> SIADYKDDDDKMRAEGLGGLERFCSPGKGRGLRALQPFQVGDLLFSCPAYAYVLTVNERGNHCEYCFTRKEGLSKCGRCKQAFYCNVECQKEDWPMHKLECSPM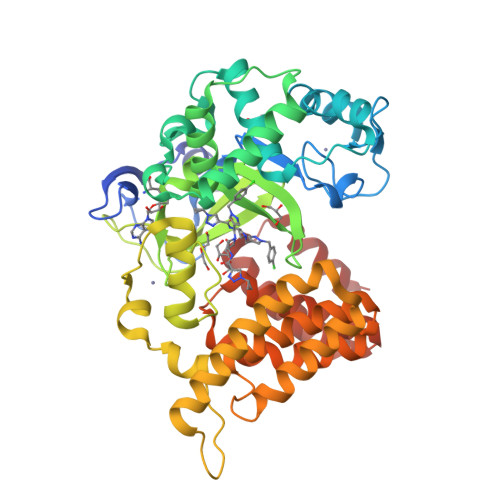VVFGENWNPSETVRLTARILAKQKIHPERTPSEKLLAVKEFESHLDKLDNEKKDLIQSDIAALHHFYSKHLGFPDNDSLVVLFAQVNCNGFTIEDEELSHLGSAIFPDVALMNHSCCPNVIVTYKGTLAEVRAVQEIKPGEEVFTSYIDLLYPTEDRNDRLRDSYFFTCECQECTTKDKDKAKVEIRKLSDPPKAEAIRDMVRYARNVIEEFRRAKHYKSPSELLEICELSQEKMSSVFEDSNVYMLHMMYQAMGVCLYMQDWEGALQYGQKIIKPYSKHYPLYSLNVASMWLKLGRLYMGLEHKAAGEKALKKAIAIMEVAHGKDHPYISEIKQEIESH> MASIDKQQIAASVPQRGFFGHPKGLFTLFFTEFWERFSYYGMRAILVYYMYYEVSKGGLGLDEHLALAIMSIYGALVYMSGIIGGWLADRVFGTSRAVFYGGLLIMAGHIALAIPGGVAALFVSMALIVLGTGLLKPNVSSIVGDMYKPGDDRRDAGFSIFYMGINLGAFLAPLVVGTAGMKYNFHLGFGLAAVGMFLGLVVFVATRKKNLGLAGTYVPNPLTPAEKKKAAAIMAVGAVVIAVLLAILIPNGWFTVETFISLVGILGIIIPIIYFVVMYRSPKTTAEERSRVIAYIPLFV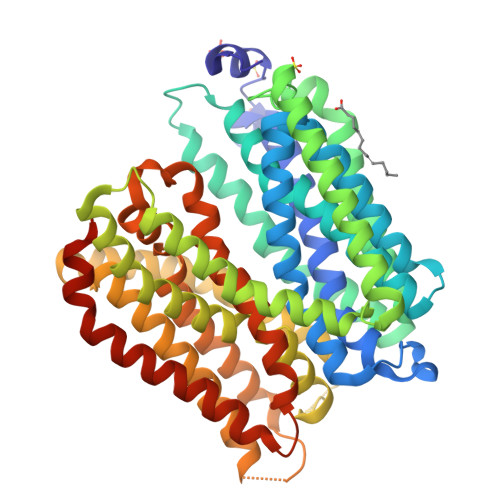ASAMFWAIQQQGSTILANYADKRTQLDVAGIHLSPAWFQSLNPLFIIILAPVFAWMWVKLGKRQPTIPQKFALGLLFAGLSFIVILVPGHLSGGGLVHPIWLVLSYFIVVLGELCLSPVGLSATTKLAPAAFSAQTMSLWFLSNAAAQAINAQLVRFYTPENETAYFGTIGGAALVLGLILLAIAPRIGRLMKGIRLESSGENLYFQ>[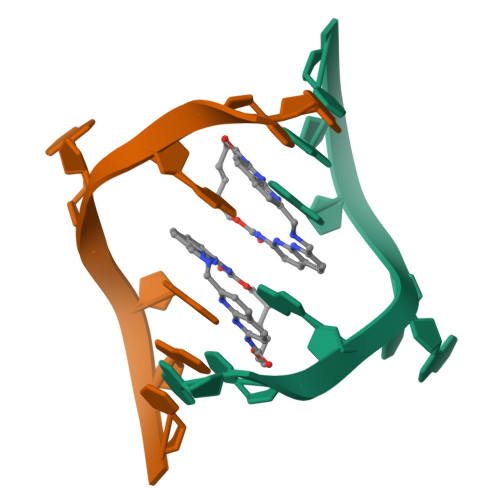4x]GCAGCAGC> RPQGATVSLWETVQKWREYRRQCQRSLTEDPPPATDLFCNRTFDEYACWPDGEPGSFVNVSCPWYLPWASSVPQGHVYRFCTAEGLWLQKDNSSLPWRDLSECEESKRGERSSPEEQLLF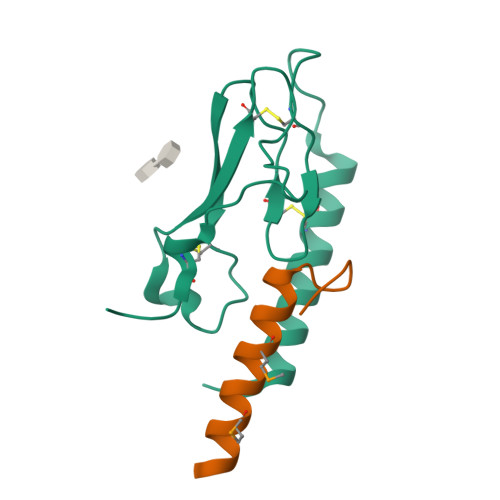LY;> DLSKQMEEEAVRMFIEWLKNGGPSSGAPPPS> GSPGIPMVAAHAAHSQSSAEWIACLDKRPLERSSEDVDIIFTRLKGVKAFEKFHPNLLRQICLCGYYENLEKGITLFRQGDIGTNWYAVLAGSLDVKVSETSSHQDAVTICTLGIGTAFGESILDNTPRHATIVTRESSELLRIEQEDFKALWEKYRQYMAGLLAPPYGVMETGSNNDRIPDKENVPSEKILRAGKI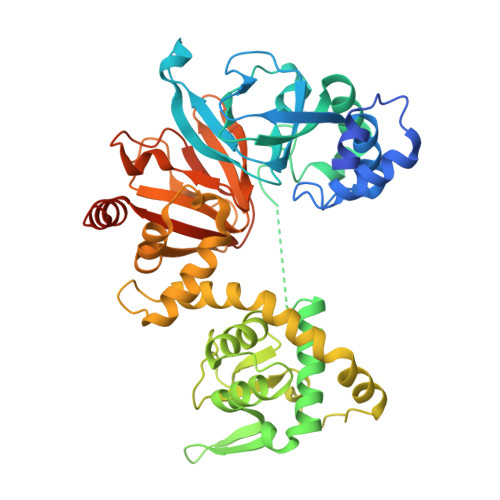LRIAILSRAPHMIRDRKYHLKTYRQCCVGTELVDWMIQQTSCVHSRTQAVGMWQVLLEDGVLNHVDQERHFQDKYLFYRFLDDEREDAPLPTEEEKKECDEELQDTMLLLSQMGPDAHMRMILRKPPGQRTVDDLEIIYDELLHIKALSHLSTTVKRELAGVLIFESHAKGGTVLFNQGEEGTSWYIILKGSVNVVIYGKGVVCTLHEGDDFGKLALVNDAPRAASIVLREDNCHFLRVDKEDFNRILRDVEANTVRLKEHDQDVLVLEKVP>[2x]GKPEAQPFAHLTINAASIPSGSHKVTLSSWYHDRGWAKISNMTLSNGKLRVNQDGFYYLYANICFRHHETSGSVPTDYLQLMVYVVKTSIKIPSSHNLMKGGSTKNWSGNSEFHFYSINVGG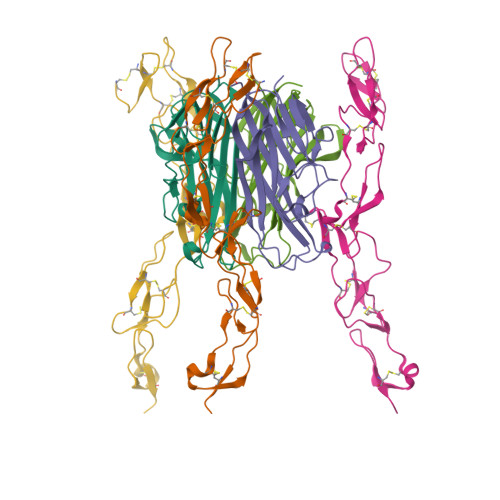FFKLRAGEEISIQVSNPSLLDPDQDATYFGAFKVQDID;>[2x]TPPCTQERHYEHLGRCCSRCEPGKYLSSKCTPTSDSVCLPCGPDEYLDTWNEEDKCLLHKVCDAGKALVAVDPGNHTAPRRCACTAGYHWNSDCECCRRNTECAPGFGAQHPLQLNKDTVCTPCLLGFFSDVFSSTDKCKPWTNCTLLGKLEAHQGTTESDVVCSSSMTL>GFQKIPVALLTTTGRKTGQPRVNPLYFLRDGGRVIVAASKGGAEKNPMWYLNLKANPKVQVQIKKEVLDLTARDATDEERAEYWPQLVTMYPSYQDYQSWTDRTIPIVVCEP[10x]

A deazaflavin-dependent nitroreductase (Ddn) from Mycobacterium tuberculosis catalyzes the reduction of nitroimidazoles such as PA-824, resulting in intracellular release of lethal reactive nitrogen species. The N-terminal 30 residues of Ddn are functionally important but are flexible or access multiple conformations, preventing structural characterization of the full-length, enzymatically active enzyme. The split barrel-like fold is characterized by a central six-stranded antiparallel β barrel in a Greek key topology with four α helices: A at the N terminus (the putative helix removed for Ddn structure determination), B after an extended loop between strands β3 and β4, and C and D between strands β5 and β6. The identification of these residues and the lack of classic catalytic residues in the active site suggest that Ddn functions primarily by precisely orienting PA-824 for efficient direct hydride transfer from F420 and potentially through additional transition-state stabilization.

Cocrystals of the NΔ40 construct with oxidized F420 were also obtained in two space groups and were solved by molecular replacement (Holo-1 in C2 at 2.1 Å resolution and Holo-2 in P21 at 1.8 Å resolution, with an rmsd for one chain of 0.3 Å over 109 aligned Cα atoms). Although the F420 preparation included larger polyglutamate tail species, only two glutamates could be visualized (F420-2), consistent with the structure of FGD1 crystallized with a similar preparation (Bashiri et al., 2008) and the recent observation that F420-2 and F420-5 bind with similar affinity to Ddn (Gurumurthy et al., 2012). The crystal packing combined with crystallographic symmetry operations reveals the same decameric ring structure in both structures, with five monomers in the ASU of Holo-1 and ten in Holo-2 (two rings per ASU). Although the decamer structure includes extensive intersubunit packing, its relevance to the native quaternary structure and function remains unknown because of the difficulties of studying the full-length enzyme. In structures Holo-1 and Holo-2, F420 binds to a groove on the surface of Ddn through a series of hydrogen bonds and several salt bridges between positive charges on Ddn and the negatively charged phosphate and tail of the coenzyme. The last visible glutamate of the F420 tail lies near the β1-β2 hairpin within hydrogen-bonding range of the side chains of R54, T56, and R60 as well as the main chain of K55 and T56. The more proximal glutamate H bonds with the side chain of N91 from helix B. The phosphate of F420 sits near the complementary positive charge of K79 and H bonds to the amides of M87 and W88 from the loop after strand β3. The deazaflavin ring system is stabilized by H bonds with the main chain of A76 and K79 and the side chain of Y133 (helix D). Additionally, there are waters in both costructures that mediate interactions between protein and coenzyme.>ADLPGSHDLDILPRFPRAEIVDFRQAPSEERIYPLGAISRISGRLRMEGEVRAEGELTALTYRLPPEHSSQEAFAAARTALLKADATPLFWCERRDCGSSSLLANAVFGNAKLYGPDEQQAYLLVRLAAPQENSLVAVYSITRGNRRAYLQAEELKADAPLAELLPSPATLLRLLKANGELTLSHVPAEPAGSWLELLVRTLRLDTGVRVELSGKHAQEWRDALRGQGVLNSRMELGQSEVEGLHLNWLR[2x]

The protein was found to be monomeric and the structure consists of two domains, domains 1 and 2, comprising residues 24–184 and 185–268, respectively. The fold of these domains could not be predicted even using state-of-the-art prediction methods, and similarity searches revealed only a very distant homology to known structures, namely to Mog1p/PsbP-like and OmpA-like proteins for the N- and C-terminal domains, respectively. Since PA1624 is only present in an important human pathogen, its unique structure and periplasmic location render it a potential drug target.

The protein was heterologously expressed in E. coli without its periplasmatic localization signal (Δ18PA1624). The data collected from the native crystal were not further used for refinement and structure analysis as the diffraction data obtained from the SeMet crystals were of higher quality. The asymmetric unit of the orthorhombic crystal form studied here contained two chains of Δ18PA1624, which superpose with a Cα r.m.s.d. of 0.5 Å, which is only slightly higher than the coordinate error. PISA analysis indicates that the protein is monomeric, which is in line with observations made during the course of purification by size-exclusion chromatography. Except for a handful of flexible residues at the N-terminus, both chains could be traced with confidence. The Δ18PA1624 monomer has approximate dimensions of 54 × 45 × 48 Å. The two domains interact through a relatively small hydrophobic interface covering about 600 Å2. The larger domain is dominated by a six-stranded antiparallel β-sheet that is covered by one α-helix on the face that also harbors the N-terminus and by a mixed α/β structure on the other. Towards this, it is interesting to note that the interior of the C-terminal domain of the protein is not optimally packed, leaving a cavity lined by hydrophobic residues unoccupied. Therefore, we suggest that PA1624 has a novel, yet-to-be-named architectural domain arrangement.>[4x]MKKWSDTE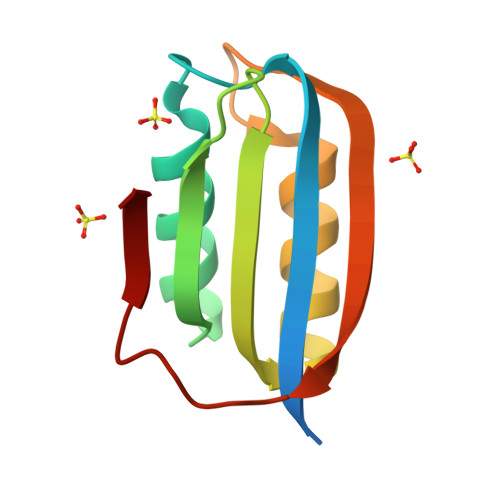VFEMLKRMYARVYGLVQGVGFRKFVQIHAIRLGIKGYAKNLPDGSVEVVAEGYEEALSKLLERIKQGPPAAEVEKVDYSFSEYKGEFEDFETY> GPLGSPGIPDSARSFLERLEARGGREGAVLAGEFSDIQACSAAWKADGVCSTVAGSRPENVRKNRYKDVLPYDQTRVILSLL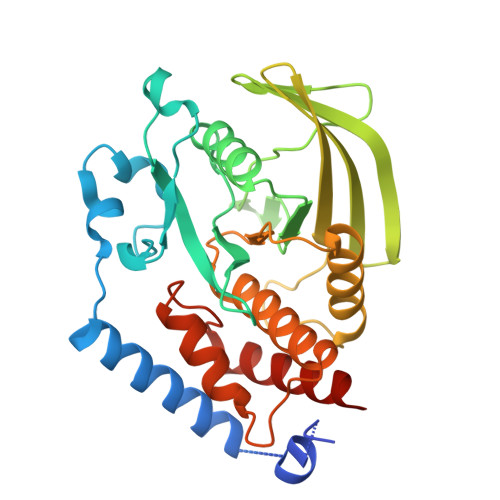QEEGHSDYINGNFIRGVDGSLAYIATQGPLPHTLLDFWRLVWEFGVKVILMACREIENGRKRCERYWAQEQEPLQTGLFCITLIKEKWLNEDIMLRTLKVTFQKESRSVYQLQYMSWPDRGVPSSPDHMLAMVEEARRLQGSGPEPLCVHCSAGCGRTGVLCTVDYVRQLLLTQMIPPDFSLFDVVLKMRKQRPAAVQTEEQYRFLYHTVAQMFCSTLQNA> MLSPPRRKAFKKWTPPRSPFNLVQETLFHDPWKLLIATIFLNRTSGKMAIPVLWKFLEKYPSAEVARTADWRDVSELLKPLGLYDLRAKTIVKFSDEYLTKQWKYPIELHGIGKY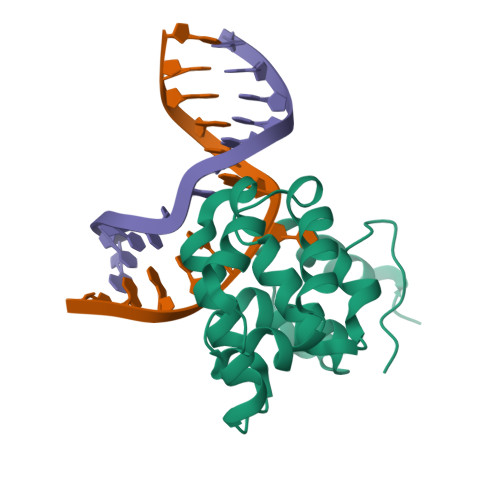GNDSYRIFCVNEWKQVHPEAHKLNKYHDWLWENHEKLSLSHHHHHH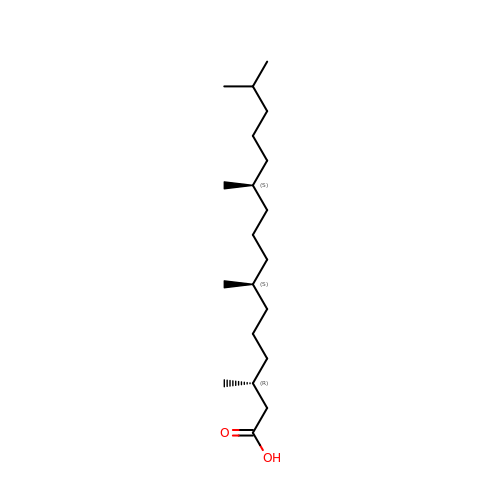(3R,7S,11S)-3,7,11,15-tetramethylhexadecanoic acid | C20 H40 O2 | RLCKHJSFHOZMDR-GBESFXJTSA-N>MKPVSLSYRCPCRFFESHIARANVKHLKILNTPNCALQIVAR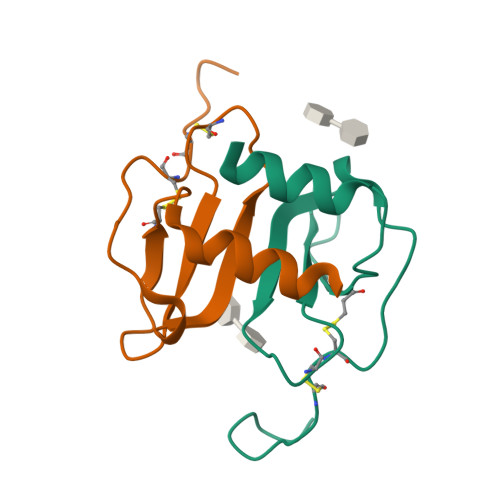LKNNNRQVCIDPKLKWIQEYLEKALN[2x]> HMKTVLMVAEKPSLAQSIAKILSRGSLSSHKGLNGACSVHEYTGTFAGQPVRFKMTSVCGHVMTLDFLGKYNKWDKVDPAELFSQAPTEKKEANPKLNMVKFLQVEGRGCDYIVLWLDCDKEGENICFEVLDAVLPVMNKAHGGEKTVFRARFSSITDTDICNAMACLGEPDHNEALSVDARQELDLRIGCAFTRFQTKYFQGKYGDLDSSLISFGPCQTPTLGFCVERHDKIQSFKPETYWVLQAKVNTDKDRSLLLDWDRVRVFDREIAQMFLNMTKLEKEAQVEATSRKEKAKQRPLALNTVEMLRVASSSLGMGPQHAMQTAERLYTQGYISYPRTETTHYPENFDLKGSLRQQANHPYWADTVKRLLAEGINRPRKGHDAGDHPPITPMKSATEAELGGDAWRLYEYITRHFIATVSHDCKYLQSTISFRIGPELFTCSGKTVLSPGFTEVMPWQSVPLEESLPTCQRGDAFPVGEVKMLEKQTNPPDYLTEAELITLMEKHGIGTDASIPVHINNICQRNYVTVESGRRLKPTNLGIVLVHGYYKIDAELVLPTIRSAVEKQLNLIAQGKADYRQVLGHTLDVFKRKFHYFVDSIAGMDELMEVSFS;> GPGHMAQVAGAALSQAGWYLSDEGIEACTSSPDKVNVNDIILIALNTDLRTIGKKFLPSDINSGKVEKLEGPCVLQIQKIRNVAAPKDNEESQAAPRMLRLQMTDGHISCTAVEFSYMSKISLNTPPGTKVKLSGIVDIKNGFLLLNDSNTTVLGGEVEHLIEKW

Topoisomerase III (TOP3) is a member of the type IA topoisomerase family, which functions mainly in relaxing the supercoiled DNA and in resolving recombination intermediates during meiosis and DNA repair. TOP3β is an atypical topoisomerase that can recognize both DNA and RNA as the substrates12132223242526. Eukaryotic TOP3α and β are unique in that they interact with their specific auxiliary factors, RMI1 and TDRD3, respectively, and coexist with them in the cell. We determined the crystal structures of human TOP3β TOPO domain, TDRD3 DUF1767 and OB domains (DUF–OB) and their complex at 3.44 Å, 1.62 Å and 3.6 Å resolutions, respectively.

Overall, the TOP3β–TDRD3 structure is similar to the TOP3α–RMI1 structure. Binding of TDRD3 did not affect the spatial arrangement of domains I, III and IV. The interaction between TOP3β and TDRD3 occurs between domain II of TOP3β and the OB-fold domain of TDRD3, consistent with our finding that the TDRD3 OB-fold domain is sufficient for binding to TOP3β. The core-mediated interaction is primarily hydrophobic: Val109, Phe111, Phe139 and Leu141 of TDRD3 and Ile269, Met272, Phe273, Met276 and Pro437 of TOP3β engage in this hydrophobic interaction. In addition, a hydrogen bond is formed between TDRD3 Arg96 and TOP3β Asp266. The insertion loop of TDRD3 interacts with the loop connecting β10 and α7 of TOP3β. In the N-terminal region of the insertion loop, Val79, Ala80, Ala81 and Pro82 of TDRD3 form a hydrophobic surface to interact with Val264, Phe265 and Ile269 of TOP3β. Furthermore, in the C-terminal region of the insertion loop, Ala90, Ala91, Pro92 and Met94 of TDRD3 also form a hydrophobic surface to interact with Val262, Val264, Ile269 and Phe273 of TOP3β. TDRD3 does not slow down the DNA relaxation activity of TOP3β32 but rather enhances it, in agreement with the short insertion loop of TDRD3, which is located far from the catalytic center composed of domains I, III and IV in the TOP3β–TDRD3 complex.>[2x]EGVSNLVGLPNNICLQKTSNQILKPKLISYTLPVVGQSGTCITDPLLAMDEGYFAYSHLERIGSCSRGVSKQRIIGVGEVLDRGDEVPSLFMTNVWTPPNPNTVYHCSAVYNNEFYYVLCAVSTVGDPILNSTYWSGSLMMTRLAVKPKSNGGGYNQHQLALRSIEKGRYDKVMPYGPSGIKQGDTLYFPAVGFLVRTEFKYNDSNCPITKCQYSKPENCRLSMGIRPNSHYILRSGLLKYNLSDGENPKVVFIEISDQRLSIGSPSKIYDSLGQPVFYQASFSWDTMIKFGDVLTVNPLVVNWRNNTVISRPGQSQCPRFNTCPEICWEGVYNDAFLIDRINWISAGVFLDS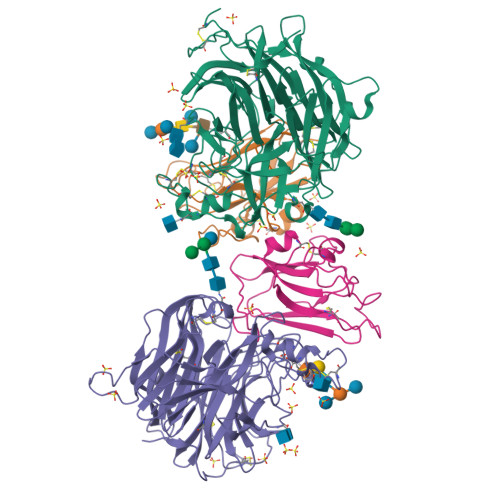NQTAENPVFTVFKDNEILYRAQLASEDTNAQKTITNCFLLKNKIWCISLVEIYDTGDNVIRPKLFAVKIPEQCTA;>[2x]SLEPVYWNSANKRFQAEGGYVLYPQIGDRLDLLCPRARPPGPHSSPSYEFYKLYLVEGAQGRRCEAPPAPNLLLTCDRPDLDLRFTIKFQEYSPNLWGHEFRSHHDYYIIATSDGTREGLESLQGGVCLTRGMKVLLRVGQ> QPIFLNVLEAIEPGVVCAGHDNNQPDSFAALLSSLNELGERQLVHVVKWAKALPGFRNLHVDDQMAVIQYSWMGLMVFAMGWRSFTNVNSAMLYFAPDLVFNEYRMHKSRMYSQCVRMRHLSQ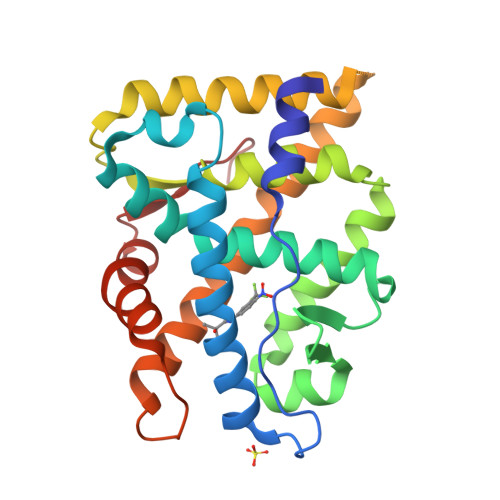EFGWLQITPQEFLCMKALLLFSIIPVDGLKNQKFFDELRMNYIKELDRIIACKRKNPTSCSRRFYQLTKLLDSVQPIARELHQFAFDLLIKSHMVSVDFPEMMAEIISVQVPKILSGKVKPIYFHTQ>GGELMIKSSNAFDVIELSSQIQRYASLSKINNRTNPILKDNKAKEFKDADLKWLKLENCPTAGDVPTTGNNNDLQDQFIACDADYRKGDLSYFGSQFEFSTYVHPSNPEIQRQIKQVVSYFQYRGMERAFIGDAAGYVISEAKKKGFSAQDYRIVLIEPDRVGYFESNAISYEEFIENPSARENFLLKATKDRTLALAVSLAQTGEIAMQRDGSVAFLEDSELCWDTAAGSAKSCLSVRYDTVGNKTELDLKQIDVVSAKGLSFESDGKTKTPVVSTYETFQDGGRAKTINAIECPTGLNNRFAAVVSSFSTAGQNANFSSESAKDSQGTTQKDGSKGPHALLSGISLNWTLTNKVWDVTASIGIESGILPTSGIDSGSLLRNPKSLSFIAFQWCEN[3x];>[3x]FNDNYSSTSTVYATSNEATDSRGSEHLRYPYLECIKIGMSRDYLENCVKVSFPTSQDMFYDAYPSTESDGAKTRTKEDFSARLLAGDYDSLQKLYIDFYLAQTTFDWEIPTRDQIETLVNYANEGKLSTALNQEYITGRFLTKENGRYDIVNVGGVPDNTPVKLPAIVSKRGLMGTTSVVNAIPNEIYPHIKVYEGTLSRLKPGGAMIAVLEYDVNELSKHGYTNLWDVQFKVLVGVPHAETGVIYDPVYEETVKPYQPSNNLT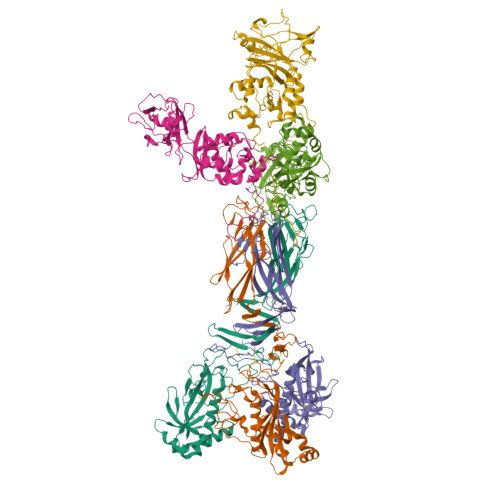GKKLYNVSTNDMHNGYKWSNTMFSNSNYKTQILLTKGDGSGVKLYSKAYSENFK>[6x]MYNDDYIEEASFLNGSDVVILIDGVEELYMEEIKADFEQDEQSIKLLGCQNEISRVGTTKGSFSLNGYKTDSKFAKLGFRSFEIIYNLSNSETLGYESIRLKNCRLKKLPLINSKAGEIVKIEVEGSFRGYDLLNEL;>[6x]MINIDRRRKDIIRTININPTNITITSIKKTEIDGAFEETETEIKCVVRIFNEKTAEKQISSEKQGTFSSIRTYGMLVSNDVILEVNSRDSLEFECIYGRMKIVNIYPQIVKGELCGYQCSLERID;>MRAGIRKALIDNIKELKGCYEPNVPNKDTKKPYMVVVQGQDNDHGETIGFERSIEVWIYEGRTTFKKLDKLTKQVVEVLDMNTIVDESENEAFTCIYKGTSENDIVVEEWDAIARGIRFSVIALEDKEDTTNDRWVEALSRHTKDLLEIESYKDNWKKNFIAPCALWRTTHIENKRINYHLIEITKTMKCHVVSKNKDEIVKLLETLETSLIIDKRVRLREDKNMYLTLVSVVEDRESDMFTTGQLTAVFKMIGKIKR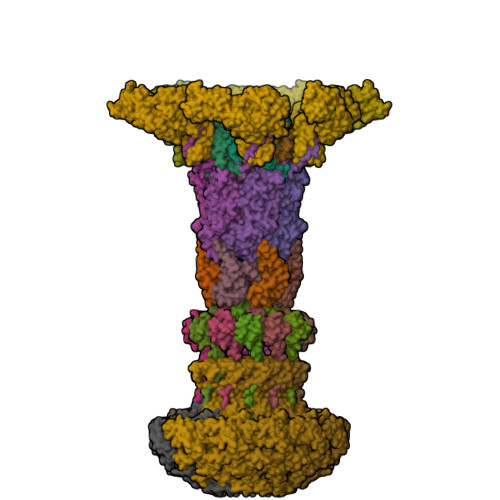EGPTMDKIYGNGNLK[6x];>[12x]MTPARDLIEKLRLLLNDKDKKSFTDEELNLFLEEADCIYCAASQGWILKSLQYENTVGEMYEYKVGQETYKSSSIKDLVSVAYQNADKFKDMCTNKKEKGSFMLGISTEFEI;>MATGTWNEKERKEIPGFYNRFKTQAEKSTNTGLKGRLAMPIRANWGDVGKVVTIKNDLRQLKNLFGDDMNYSAFKLGKLALLGNVKELLLYRLVDGNQKKGTLTLKDTTENSAKDVIKLETKYPTARNFNVTIKSNLVDSDKKDFIFFENTKQLFSSSIKGTIDEIVLEINSNLDNEYVIATKVADSDTILANVVNQALEGGNDGCTSITNESYLKALEEFERYSFDSFVLDGVADEALQETTKAWVAKNKELGKDILLFLGGKTEDNIKQINDKSKSFNDENIVNVGSSAYYENIKYTPSEVAVYIAALSVSKGITGSICNAKTIFEEVEPRLSQSEVKECLKSGTLVLDFDDGDVIIVDDVNTFKKYVDDKNEAMGYISNIMFINTINKDTSLKRKEFVGKIFNDATGQTTVICALKKYFEELMSQGIISEFNVDIDTELQATAKADEFYWKWDAVKVDVMKKIYGTGYLG[6x];>MGIISYVKKLFKRPAGEIMRMSSGNIGVYKLDDSRVDYELARELYQNKNANYKLGSSFVRPIVNSTTGFMGVPHFQIEDEEAQYILDEFVLDNTSKMLKTHTDSLKQGDCYIWITREERENPLYPDKKVRLIYNFISPEEVKEIILDPTTKEPIAYILESQNEWTDLGENKRKAKVKQIITAESRFVEVEGDKIEGLEEGETPNVWGFIPIIHFKNEADETLKYGQSDIEPIEPLLKAYHDVMLHALKGSKMHSTPKLKLKLTDVASFLAHNFGVEDPVKFAKEGGKINLDGHEILFLNKDEEAEFVEVKSAIGDAKELLKLLFYCIVDVSETPEFIFGVHTPSALASVKEQMPIMVNKIRRKREQFTNSWQLLARMVLIMSSNSSGMKYSSYDVTIGWDEVNPRDDKELAETLEKVCCALDKALEGGFISEESTVNFLAQYIDTMSNYISDDGEREGEREKIIKTKMLKYRLDDSQGLNDESNEIEKEINKIKDNNGNG[12x]> VPISPIETVPVKLKPGMDGPKVKQWPLTEEKIKALVEICTEMEKEGKISKIGPENPYNTPVFAIKKKDSTKWRKLVDFRELNKRTQDFWEVQLGIPHPAGLKKKKSVTVLDVGDAYFSVPLDEDFRKYTAFTIPSINNETPGIRYQYNVLPQGWKGSPAIFQSSMTKILEPFAAQNPDIVIYQYMDDLYVGSDLEIGQHRTKIEELRQHLLRWGLTTPDKKHQKEPPFLWMGYELHPDKWTVQPIVLPEKDSWTVNDIQKLVGKLNWASQIYPGIKVRQLSKLLRGTKALTEVIPLTEEAELELAENREILKEPVHGVYYDPSKDLIAEIQKQGQGQWTYQIYQEPFKNLKTGKYARMRGAHTNDVKQLTEAVQKITTESIVIWGKTPKFKLPIQKETWETWWTEYWQATWIPEWEFVNTPPLVKLWYQLEK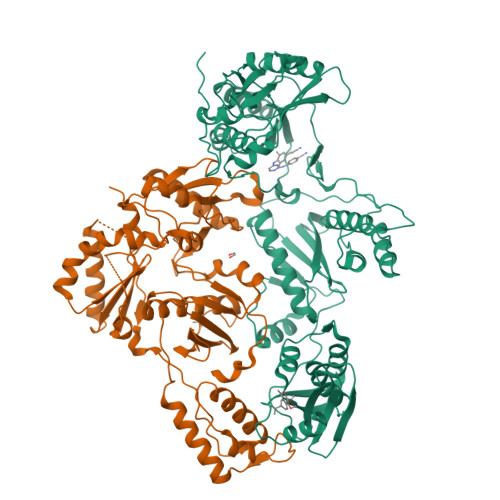EPIVGAETFYVDGAANRETKLGKAGYVTNKGRQKVVPLTNTTNQKTELQAIYLALQDSGLEVNIVTDSQYALGIIQAQPDKSESELVNQIIEQLIKKEKVYLAWVPAHKGIGGNEQVDKLVSA;> ETVPVKLKPGMDGPKVKQWPLTEEKIKALVEICTEMEKEGKISKIGPENPYNTPVFAIKKKDSTKWRKLVDFRELNKRTQDFWEVQLGIPHPAGLKKKKSVTVLDVGDAYFSVPLDEDFRKYTAFTIPSINNETPGIRYQYNVLPQGWKGSPAIFQSSMTKILEPFKKQNPDIVIYQYMDDLYVGSDLEIGQHRTKIEELRQHLLRWGLTTPDKKHQKEPPFLWMGYELHPDKWTVQPIVLPEKDSWTVNDIQKLVGKLNWASQIYPGIKVRQLSKLLRGTKALTEVIPLTEEAELELAENREILKEPVHGVYYDPSKDLIAEIQKQGQGQWTYQIYQEPFKNLKTGKYARMRGAHTNDVKQLTEAVQKITTESIVIWGKTPKFKLPIQKETWETWWTEYWQATWIPEWEFVNTPPLVKLWYQ(1S)-1,5-anhydro-1-[5-(naphthalen-2-yl)-1H-imidazol-2-yl]-D-glucitol 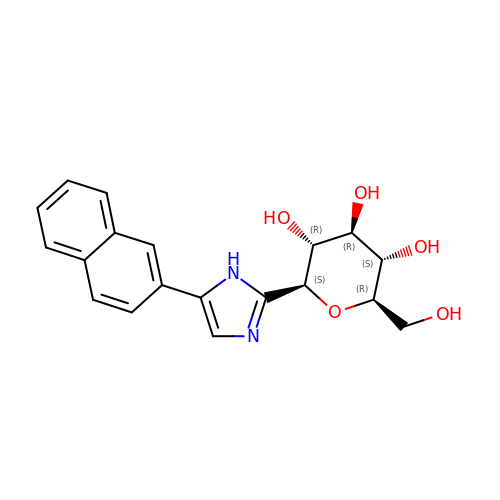| C19 H20 N2 O5 | AXGMUNPLTDCCLX-UYTYNIKBSA-N TrkH, KtrB, and more distantly related KdpA belong to the superfamily of K+ transporters (SKTs) that are found in bacteria, fungi, and plants. TrkH or KtrB proteins assemble with their respective cytosolic partner proteins TrkA or KtrA to form a stable complex. To better understand the mechanism by which the Trk system functions, we determined the structures of TrkH-TrkA complex from V. parahaemalyticus in the presence of ADP (TrkHA-ADP), ATP (TrkHA-ATP), or ATPγS (TrkHA-ATPγS).

As an alternative approach to visualize ligand-induced structural changes in TrkA, we solved the structure of the TrkHA complex in the presence of an ATP analog, ATPγS, to 3.85 Å resolution by X-ray crystallography (TrkHA-ATPγS, Rwork/Rfree = 0.27/0.33). The TrkHA protein was crystallized in the presence of 10 mM of ATPγS. TrkA remains a tetramer; however, the shape of the tetramer is different from that of the TrkHA-ADP. TrkH remains a dimer and is in the closed state, and while the HN2 interface is preserved, the extent of the HN1 interface is significantly reduced. The N2 domain has a 20° rotation relative to the N1 domain when compared to the structure of a TrkA in the presence of ADP. Although relatively small, the rotation of the N2 domain in the ATPγS bound TrkA is sufficient to break the bulk of the N2-N2 interface so that there is only a tenuous connection between the two domains. Similarly, the N1 domain is pulled away from TrkH and as a result, the HN1 interface is significantly reduced. In the TrkHA-ADP structure, ADP is only found in the N2 domain of TrkA, while in the TrkHA-ATPγS structure, ATPγS is found in both the N1 and N2 domains. In the N1 binding site, conserved residues of ASN74 interact with the adenosine ring, ASN31 interacts with the ribose, and ARG98 and ARG100 form salt bridges with the γ- and β-phosphate, respectively. TrkH protomers from the TrkHA-ATPγS are in a closed state and each protomer aligns well to that from the TrkHA-ADP; however, the TrkH dimer interface is almost identical to that of the TrkH from TrkHA-ATP.

>MQFRSIIRIVGLLLALFSVTMLAPALVALLYRDGAGVPFVTTFFVLLFCGAMCWFPNRRHKHELKSRDGFLIVVLFWTVLGSAGSLPFLIADNPNISVTDAFFESFSALTTTGATVIVGLDELPKAILFYRQFLQWFGGMGIIVLAVAILPVLGIGGMQLYRAEIPGPVKDTKMTPRIAETAKALWYIYLSLTIACAVAFWLAGMTPFDAISHSFSTIAIGGFSTHDASMGYFDSYAINLITVVFLLISACNFTLHFAAFASGGVHPKYYWKDPEFRAFIFIQVLLFLVCFLLLLKHHSYTSPYDAFDQALFQTVSISTTAGFTTTGFADWPLFLPVLLLFSSFIGGCAGSTGGGMKVIRILLLTLQGARELKRLVHPRAVYTIKVGGSALPQRVVDAVWGFFSAYALVFVVCMLGLIATGMDELSAFSAVAATLNNLGPGLGEVALHFGDVNDKAKWVLIVSMLFGRLEIFTLLILLTPTFWRS[2x];>[2x]MKIIILGAGQVGGTLAENLVGENNDITIVDNNADRLRELQDKYDLRVVNGHASHPDVLHEAGAQDADMLVAVTNTDETNMAACQVAFTLFNTPNRVARIRSPEYLAEKEALFKSGAIPVDHLIAPEELVTSYIERLIQYPGALQVVSFAEQKVSLVAVKAYYGGPLVGNALSALREHMPHIDTRVAAIFRQGRPIRPQGTTIIEADDEVFFVAASNHIRSVMSELQRLEKPYRRIMIVGGGNIGASLAKRLEQTYSVKLIERDYQRAEKLSEQLENTIVFCGDAADQELLTEENIDQVDVFIALTNEDETNIMSAMLAKRMGAKKVMVLIQRGAYVDLVQGGVIDVAISPQQATISALLTHVRRADIVNVSSLRRGAAEAIEAVAHGDETTSKVVGRAIGDIKLPPGTTIGAVVRGEEVLIAHDRTVIEQDDHVVMFLVDKKYVPDVEALFQPSPFFL> CHLSDLLQQLTSVNASKPSERGLVRQEEAEDPACIPIFWVSKWVDYSDKYGLGYQLCDNSVGVLFNDSTRLILYNDGDSLQYIERDGTESYLTVSSHPNSL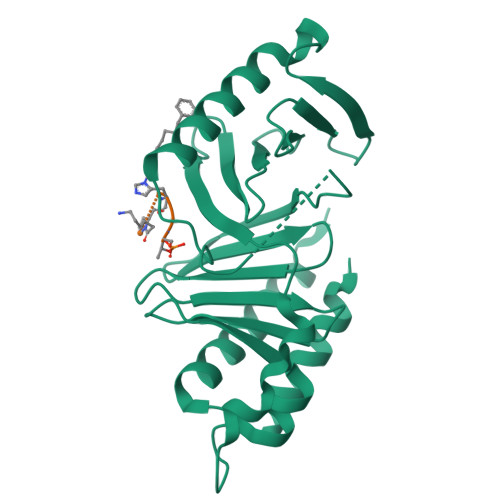MKKITLLNYFRNYMSEHLLKAGANITPREGDELARLPYLRTWFRTRSAIILHLSNGTVQINFFQDHTKLILCPLMAAVTYINEKRDFQTYRLSLLEEYGCCKELASRLRYARTMVDKLLSSRS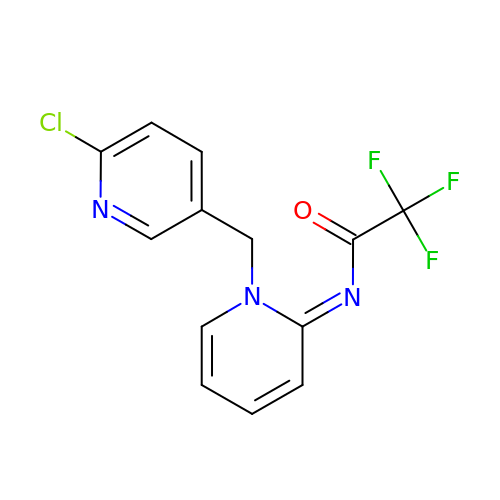(~{N}~{E})-~{N}-[1-[(6-chloranylpyridin-3-yl)methyl]pyridin-2-ylidene]-2,2,2-tris(fluoranyl)ethanamide | C13 H9 Cl F3 N3 O | DHQKLWKZSFCKTA-YBFXNURJSA-N[5-(4-fluoro-2H-isoindole-2-carbonyl)-2-hydroxyphenyl](5-fluoro-2H-isoindol-2-yl)methanone 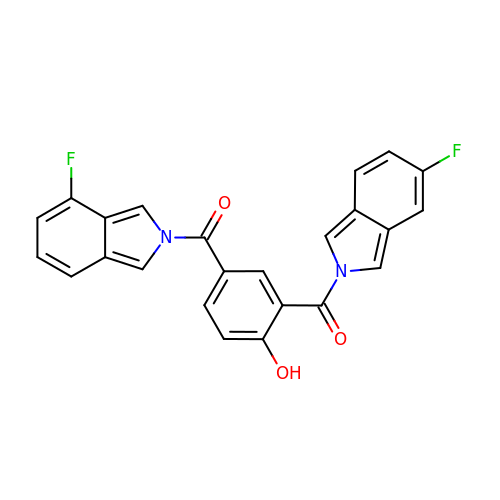| C24 H14 F2 N2 O3 | NDSVVWMRIUKJHF-UHFFFAOYSA-N> IPEGILMEKNNVDIAEGQGYSLDQEAGAKYVKAMTQGTIILSYKSTSENGIQSLFSVGNSTAGNQDRHFHIYITNSGGIGIELRNTDGVFNYTLDRPASVRALYKGERVFNTVALKADAANKQCRLFANGELLATLDKDAFKFISDITGVDNVTLGGTKRQGKIAYPFGGTIGDIKVYSNALSDEELIQATGVTTYGENIFYAGDVTESNYFRIPSLLTLSTGTVISAADARYGGTHDSKSKINIAFAKSTDGGNTWSEPTLPLKFDDYIAKNIDWPRDSVGKNVQIQGSASYIDPVLLEDKLTKRIFLFADLMPAGIGSSNASVGSGFKEVNGKKYLKLRWHKDAGRAYDYTIREKGVIYNDATNQPTEFRVDGEYNLYQHDTNLTCKQYDYNFSGNNLIESKTDVDVNMNIFYKNSVFKAFPTNYLAMRYSDDEGASWSDLDIVSSFKPEVSKFLVVGPGIGKQISTGENAGRLLVPLYSKSSAELGFMYSDDHGDNWTYVEADNLTGGATAEAQIVEMPDGSLKTYLRTGSNCIAEVTSIDGGETWSDRVPLQGISTTSYGTQLSVINYSQPIDGKPAIILSSPNATNGRKNGKIWIGLV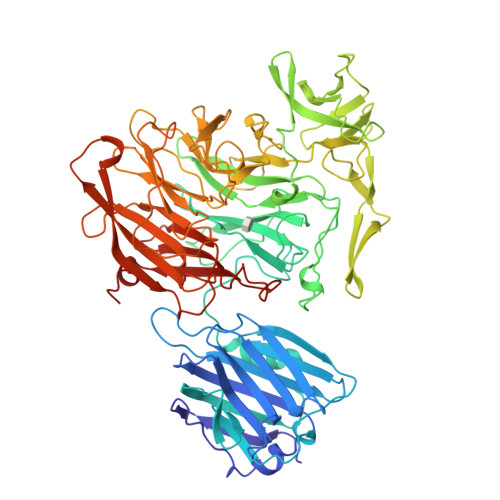NDTGNTGIDKYSVEWKYSYAVDTPQMGYSYSCLAELPDGQVGLLYEKYDSWSRNELHLKDILKFEKYSISELTGQA> AGAGAAGAAAGGGAAAUUUUUUUUUUUUUUUU

We compared the direct-methods structure determination of a double-stranded RNA (dsRNA; 32 base pairs, one strand in the asymmetric unit, 675 non-H atoms, two levels of imperfect TPS) with that of a single-stranded RNA (ssRNA) hairpin (27 nucleotides, one strand in the asymmetric unit, 580 non-H RNA atoms, no TPS). The dsRNA is a pathological case for ab initio structure determination in the presence of TPS and the hairpin is a case for ab initio structure determination by direct methods in the absence of TPS. The ab initio structure-determination experiments were performed with the direct-methods program SIR2014, which uses dual-space methods to attempt structure determination from random phases. The pmf for the dsRNA was broader than that for the hairpin and the mean number of trials was almost six times larger.

Using direct methods starting from random phases, the crystal structure of a 32-base-pair RNA (675 non-H RNA atoms in the asymmetric unit) was determined using only the native diffraction data (resolution limit 1.05 Å) and the computer program SIR2014. The 32 nt dsRNA was a head-to-head fusion of two U-helices from a RNA-editing substrate from trypanosomes. The 3′ half of the fusion RNA consisted of 16 consecutive Us that represented the U-tail of the guide RNA. This tail formed ten A–U Watson–Crick base pairs and six G–U wobble base pairs with the 5′ half of the fusion RNA. The 5′ half represented the purine-rich pre-edited mRNA. The RNA was one base pair short of the 33 base pairs required for three helical turns in A-form RNA (11 base pairs per turn). Three double helices stacked end-on-end along the c edge of the R32:H unit cell. The almost three helical turns of the RNA in the asymmetric unit introduced partial or imperfect translational pseudosymmetry (TPS) that modulated the intensities when averaged by the l Miller indices but still escaped automated detection. The z coordinate was arbitrary for the hairpin in P43. The z components of the shift vectors for the dsRNA were zero (the correct value because the molecular dyad sits on a crystallo­graphic twofold) for about one eighth of the trials but had different values for the remaining trials.(4~{S})-4-[4-[bis(fluoranyl)methoxy]-3-methyl-phenyl]-4-[3-(5-chloranylpyridin-3-yl)phenyl]-5~{H}-1,3-oxazol-2-amine | C22 H18 Cl F2 N3 O2 | 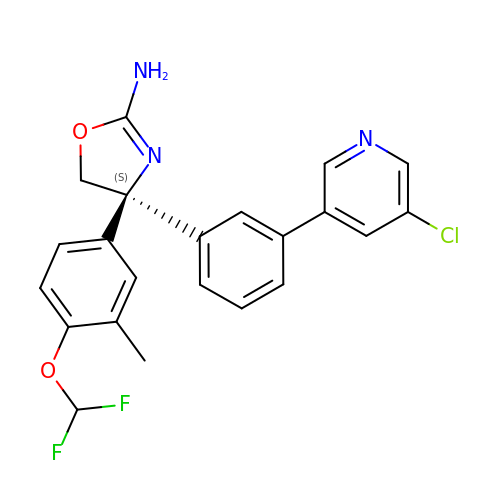UQLVXWKMSVKVGL-QFIPXVFZSA-N>[2x]NTQLMGE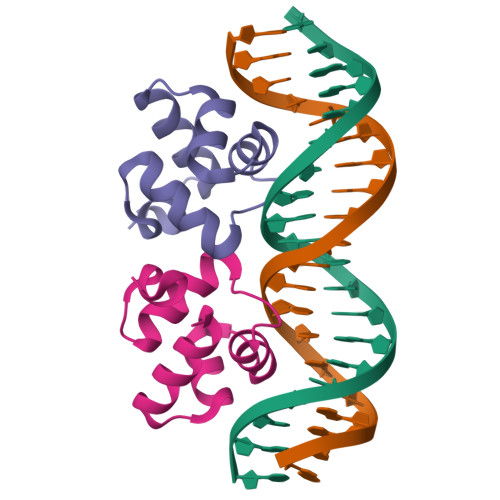RIRARRKKLKIRQAALGKMVGVSNVAISQWERSETEPNGENLLALSKALQCSPDYLLKGD> MQPSQVSNNGPMPGHPRLLLLSGEEDALKRTISADKTWEKLHQAIVAECDQLVGIEPLKRIQIGRRLLDKSREALRRIFYLSYAWRMTHQLNYLQRAETELLTIAAFSDWNPTHFLDVAEMTMAVSIGYDWLYNDLSEQSRSTIKEAILKKGIEPSMDSKYNSWLRSSNNWNQVCNAGITYGAIAVYEDQPEQSKALISRAVSAVVLPMGDYKPDGAYPEGYSYWGYGTSFNVMLISALDKLFGNDFGLSAQPGFLKTAGYLENMTAPSGNAYNYSDSGLSGELQPAMFWFAKKLNDPSLLWVERSRLMNSNPQNHLRNRLLPAALLWSNGVKVAQMNAPKEAMWVGEGKTPVALMRTSWTDPAAIFVGMKGGSPGTSHAHMDVGSFVMEADGVRWAMDFGMQEYESLESKGVDLWNMKQNSQRWQILRYNNFAHNTLSINDELQAVDGKAPLTAHSSSANFMNAQVDLSSLYKQSIAKANRGIAVVDKAYVVVQDEIETSPAEATVRWTLLTSATVKVTGANQAELTKDGKVLTIQVMEPAQIDFKTWPTEPVYDFDAPNPGTTLVGFEVKLPANTKSVIQVTLTPGSSAGQKKKPVEPLSQWPRLEHHHHHH

Recently, a new class of glycosaminoglycan (GAG) lyases (GAGases) belonging to PL35 family has been discovered with an ultrabroad substrate spectrum that can degrade three types of uronic acid-containing GAGs (hyaluronic acid, chondroitin sulfate and heparan sulfate) or even alginate. In this study, crystal structures of two GAGases (GAGase II and GAGase VII) were determined for the first time, and their catalytic mechanism was further elucidated through the site-directed mutagenesis of their crucial site residues and molecular docking. The structures of GAGase II from Spirosoma fluviale (GenBank accession number: SOD82962.1, 81.2% sequence identity with GAGase I), GAGase VII from Bacteroides intestinalis (GenBank accession number: EDV05210.1, 44.8% sequence identity with GAGase I) and selenomethionine (SeMet)-labeled GAGase II (Se-GAGase II) in their ligand-free states were solved at 1.9 Å, 2.4 Å, and 2.0 Å resolution, respectively. Both GAGase II and GAGase VII are monomers consisting of two domains: an N-terminal (α/α)6 toroid domain and a C-terminal two-layered β-sheet domain. Notably, GAGases are more structurally similar to alginate lyases from PL15, PL17, and PL39 family than to various GAG lyases, which further structurally supports the speculation that GAGases originated from alginate lyases.

The N-terminal domain (Met34-Ala365) of GAGase II is composed of 16 large or small α-helices (α1-α16) to form an (α/α)6 toroid domain. The C-terminal domain (Met366-Ser612) of GAGase II is composed of 17 β-strands (β1-β17) to form a two-layered β-sheet domain with four small α-helices located between β5-β6 and β8-β9. Subsequently, there is an Ω-loop structure wrapping around a metal ion (Mn2+), which consists of three small α-helices and small β-strands, with many residues (such as His401, His403, Tyr427, Glu431, Trp438, Arg446, and so on) on top, which might serve as potential substrate-binding sites. Structurally, the Mn2+ is located inside the long Ω loop after the β1-β5 antiparallel β-sheet, and coordinates with the nearby nitrogen and oxygen atoms of several residues such as Asp and His in both GAGase VII and GAGase II (GAGase II also has coordination with three surrounding water molecules), with distances of 2.0–2.5 Å. To investigate the roles of these adjacent residues interacting with the Mn2+, His403, Asp405, Asp421, and His457 in GAGase II were individually mutated to alanine (Ala), and the results showed that these variants resulted in complete or substantial inactivation of GAGase II. Compared with structurally similar GAG/alginate lyases, the results from molecular docking and catalytic tunnel predictions showed that GAGase II contains a shorter catalytic cavity, which may explain why they can accommodate and degrade a variety of substrates with very different structures.(1R,2R,3S,4S,5R)-5-AMINOCYCLOPENTANE-1,2,3,4-TETROL | C5 H11 N O4 | 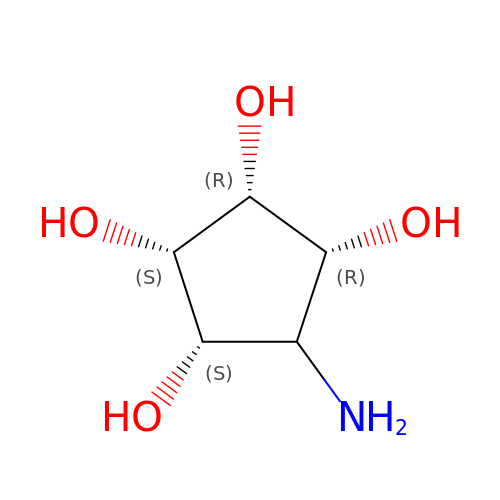LZCRRHQKPAEPKL-CTPMEXECSA-N3-{[(E)-1-carboxy-2-phenylethenyl]oxy}-2-hydroxybenzoic acid 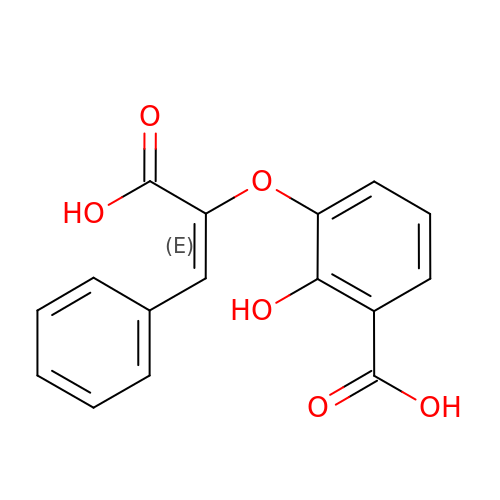| C16 H12 O6 | GJZVTQNBNWGGSJ-UKTHLTGXSA-N> IQMKRDKI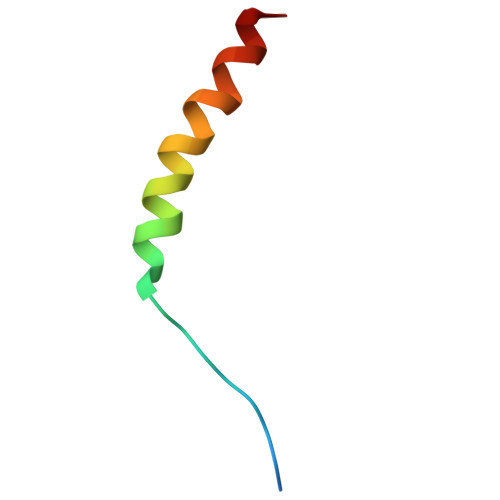KEEEQKKKEWINQERQKTLQRLRSFK>[2x]EARGATEEPSPPSRALYFSGRGEQLRLRADLELPRDAFTLQVWLRAEGGQRSPAVITGLYDKCSYISRDRGWVVGIHTISDQDNKDPRYFFSLKTDRARQVTTINAHRSYLPGQWVYLAATYDGQFMKLYVNGAQVATSGEQVGGIFSPLTQKCKVLMLGGSALNHNYRGYIEHFSLWKVARTQREILSDMETHGAHTALPQLLLQENWDNVKHAWSPMKDGSSPKVEFSNAHGFLLDTSLEPPLCGQTLCDNTEVIASYNQLSSFRQPKVVRYRVVNLYEDDHKNPTVTREQVDFQHHQLAEAFKQYNISWELDVLEVSNSSLRRRLILANCDISKIGDENCDPECNHTLTGHDGGDCRHLRHPAFVKKQHNGVCDMDCNYERFNFDGGECCDPEITNVTQTCFDPDSPHRAYLDVNELKNILKLDGSTHLNIFFAKSSEEELAGVATWPWDKEALMHLGGIVLNPSFYGMPGHTHTMIHQIGHSLGLYHVFRGISEIQSCSDPCMETEPSFETGDLCNDTNPAPKHKSCGDPGPGNDTCGFHSFFNTPYNNFMSYADDDCTDSFTPNQVARMHCYLDLVYQGWQPSRKPAPVALAPQVLGHTTDSVTLEWFPPIDGHFFERELGSACHLCLEGRILVQYASNASSPMPCSPSGHWSPREAEGHPDVEQPCKSSVRTWSPNSAVNPHTVPPACPEPQGCYLELEFLY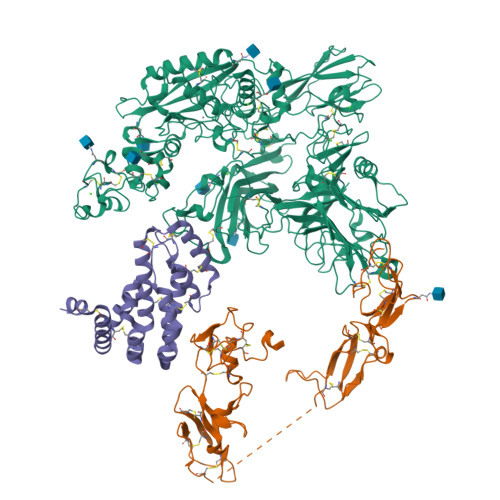PLVPESLTIWVTFVSTDWDSSGAVNDIKLLAVSGKNISLGPQNVFCDVPLTIRLWDVGEEVYGIQIYTLDEHLEIDAAMLTSTADTPLCLQCKPLKYKVVRDPPLQMDVASILHLNRKFVDMDLNLGSVYQYWVITISGTEESEPSPAVTYIHGSGYCGDGIIQKDQGEQCDDMNKINGDGCSLFCRQEVSFNCIDEPSRCYFHDGDGVCEEFEQKTSIKDCGVYTPQGFLDQWASNASVSHQDQQCPGWVIIGQPAASQVCRTKVIDLSEGISQHAWYPCTISYPYSQLAQTTFWLRAYFSQPMVAAAVIVHLVTDGTYYGDQKQETISVQLLDTKDQSHDLGLHVLSCRNNPLIIPVVHDLSQPFYHSQAVRVSFSSPLVAISGVALRSFDNFDPVTLSSCQRGETYSPAEQSCVHFACEKTDCPELAVENASLNCSSSDRYHGAQCTVSCRTGYVLQIRRDDELIKSQTGPSVTVTCTEGKWNKQVACEPVDCSIPDHHQVYAASFSCPEGTTFGSQCSFQCRHPAQLKGNNSLLTCMEDGLWSFPEALCELMCLAPPPVPNADLQTARCRENKHKVGSFCKYKCKPGYHVPGSSRKSKKRAFKTQCTQDGSWQEGACVPVTCDPPPPKFHGLYQCTNGFQFNSECRIKCEDSDASQGLGSNVIHCRKDGTWNGSFHVCQEMQGQCSVPNELNSNLKLQCPDGYAIGSECATSCLDHNSESIILPMNVTVRDIPHWLNPTRVERVVCTAGLKWYPHPALIHCVKGCEPFMGDNYCDAINNRAFCNYDGGDCCTSTVKTKKVTPFPMSCDLQGDCACRDPQAQEHS;> RLSLQNTAEIQHCLVNAGDVGCGVFECFENNSCEIRGLHGICMTFLHNAGKFDAQGKSFIKDALKCKAHALRHRFGCISRKCPAIREMVSQLQRECYLKHDLCAAAQENTRVIVEMIHFKDLLLHEPYVDLVNLLLTCGEEVKEAITHSVQVQCEQNWGSLCSILSF>[2x]SNAIRPTIGQQMETGDQRFGDLVFRQLAPNVWQHTSYLDVPGFGAVASNGLIVRDGGRVLVVDTAWTDDQTAQILNWIKQEINLPVALAVVTHAHQDKMGGMD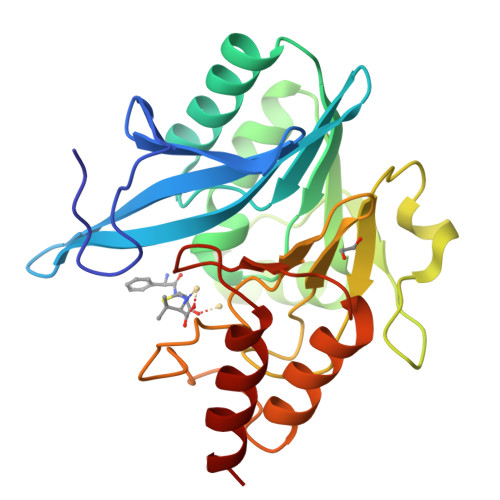ALHAAGIATYANALSNQLAPQEGMVAAQHSLTFAANGWVEPATAPNFGPLKVFYPGPGHTSDNITVGIDGTDIAFGGCLIKDSKAKSLGNLGDADTEHYAASARAFGAAFPKASMIVMSHSAPDSRAAITHTARMADKLR> GSAKDPMKQAILYVGHGSRVKKAQQEAAAFLEGCKAHVSAPVQEISFLELQEPTIETGFEACVKQGATHIAVVPLLLLTAAHAKHDIPEEIARAASRYPSIRISYGKPIG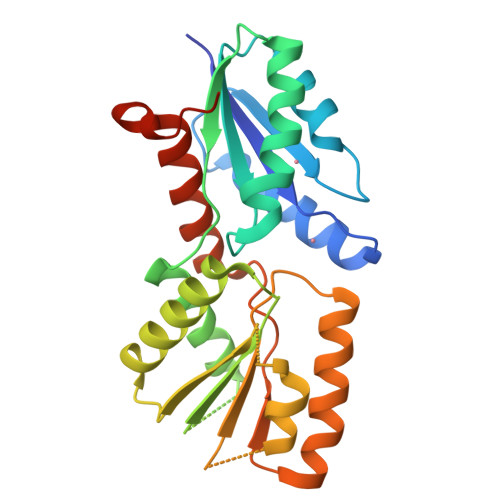IDEEVVKAVYHRMKDIGVPYENARVVLIGRGSSDPDVKRDVTGIANLLQNMIPVKEVIPCFLTACGPNYKEVLSELKKDDGVTTFVVPYLLFTGMLMNEIEREVQTLKADNPNVYLSSYIGFHPHVKNAFLNRVRETAENPEGQFDFDGGSYAPAAH> TTCCPSIVAKS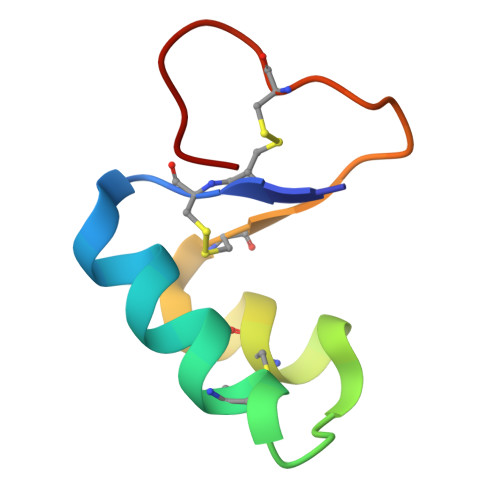NFNACRLPGTPEALCATYTGCIIIPGATCPGDYAN> VVGGTEAQ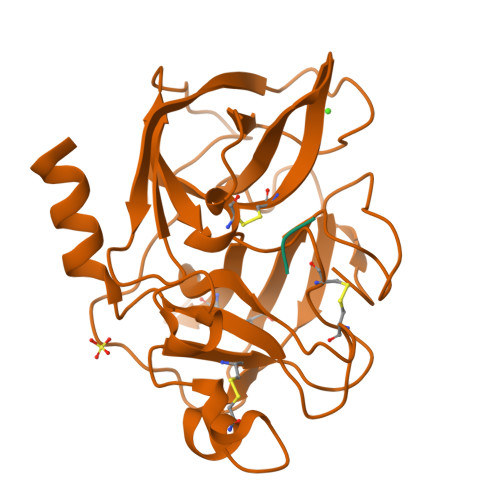RNSWPSQISLQYRSGSSWAHTCGGTLIRQNWVMTAAHCVDRELTFRVVVGEHNLNQNNGTEQYVGVQKIVVHPYWNTDDVAAGYDIALLRLAQSVTLNSYVQLGVLPRAGTILANNSPCYITGWGLTRTNGQLAQTLQQAYLPTVDYAICSSSSYWGSTVKNSMVCAGGDGVRSGCQGDSGGPLHCLVNGQYAVHGVTSFVSRLGCNVTRKPTVFTRVSAYISWINNVIASN;> YPFVEPIRF> MKEKIRKKILLAPEEPGVYIFKNKGVPIYIG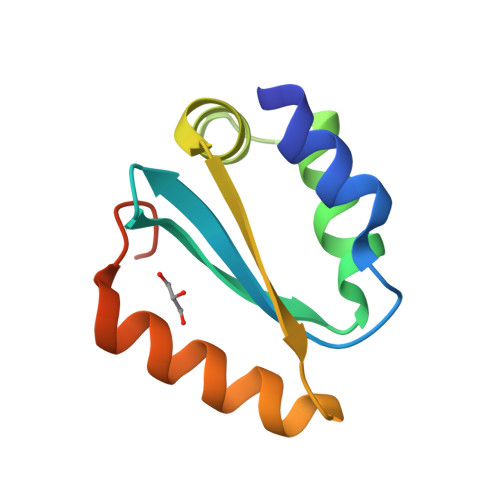KAKRLSNRLRSYLNPQTEKVFRIGEEADELETIVVMNEREAFILEANLIKKYRPKYNVRLKDTDF>[11x]MASWSHPQFEKIEGRMSVTVPNDDWTLSSLSETFDDGTQTLQGELTLALDKLAKNPSNPQLLAEYQSKLSEYTLYRNAQSNTVKVIKDVDAAIIQNFR;>MLSDMSLIATLSFFTLLPFLVAAGTCYIKFSIVFVMVRNALGLQQVPSNMTLNGIALIMALFVMKPIIEAGYENYLNGPQKFDTISDIVRFSDSGLMEYKQYLKKHTDLELARFFQRSEEENADLKSAENNDYSLFSLLPAYALSEIKDAFKIGFYLYLPFVVVDLVISSILLALGMMMMSPITISVPIKLVLFVALDGWGILSKALIEQYINIPA[5x];> MDISSWFESIHVFLILLNGVFFRLAPLFFFLPFLNNGIISPSIRIPVIFLVASGLITSGKVDIGSSVFEHVYFLMFKEIIVGLLLSFCLSLPFWIFHAVGSIIDNQRGATLSSSIDPANGVDTSELAKFFNLFSAVVFLYSGGMVFILESIQLSYNICPLFSQCSFRISNILTFLTLLASQAVILASPVMIVLLLSEVLLGVLSRFA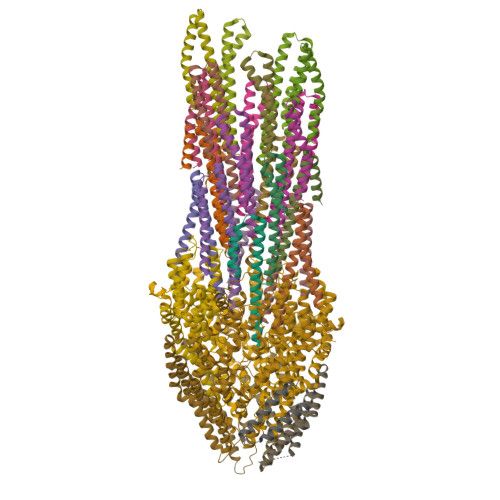PQMNAFSVSLTIKSLLAIFIIFICSSTIYFSKVQFFLGEHKFFTNLFVR;>[5x]MSDIVYMGNKALYLILIFSLWPVGIATVIGLSIGLLQTVTQLQEQTLPFGIKLIGVSISLLLLSGWYGEVLLSFCHEIMFLIKSGV> GSPAKIKIVAPLESALIPGGETYQLRCDIMSTPAATIHWKFNGKLIQGSNELNVEEKLLNFGK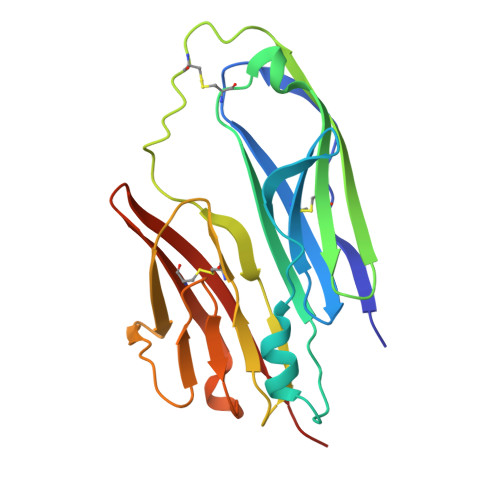AIVDTGIVASILTIQCPSAENSGTYSCVGYNGHQTIETVAEVEIEGEASGCRSNHKSAPEIVFWTDSRFEMTGNVATLVCRANQQVDWVWMSNDELVKNNDKFTVLSNGDLVIKNIVWDDMGTYTCIARNQFGEARQETFLYPTAHHHHHH>PLGSKLLLMGRSGSGKSSMRSIIFSNYSAFDTRRLGATIDVEHSHLRFLGNMTLNLWDCGGQDVFMENYFTKQKDHIFQMVQVLIHVFDVESTEVLKDIEIFAKALKQLRKYSPDAKIFVLLHKMDLVQLDKREELFQIMMKNLSETSSEFGFPNLIGFPTSIWDESLYKAWSQIVCSLIPNMSNHQSNLKKFKEIMNALEIILFERTTFLVICSSNGENSNENHDSSDNNNVLLDPKRFEKISNIMKNFKQSCTKLKSGFKTLILNNNIYVSELSSNMVCFIVLKDMNIPQELVLENIKKAKEFFQ[2x];>MVLLMGVRRCGKSSICKVVFHNMQPLDTLYLESTSNPSLEHFSTLIDLAVMELPGQLNYFEPSYDSERLFKSVGALVYVIDSQDEYINAITNLAMIIEYAYKVNPSINIEVLIHKVDGLSEDFKVDAQRDIMQRTGEELLELGLDGVQVSFYLTSIFDHSIYEAFSRIVQKLIPELSFLENMLDNLIQHSKIEKAFLFDVNSKIYVSTDSNPVDIQMYEVCSEFIDVTIDLFDLYKAPVLRNSQKSSDKDNVINPRNELQNVSQLANGVIIYLRQMIRGLALVAIIRPNGTDMESCLTVADYNIDIFKKGLED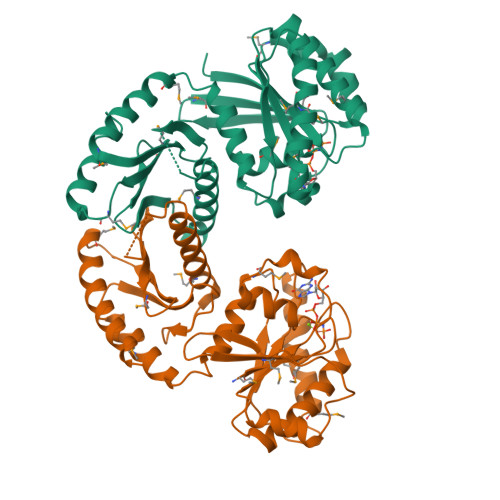IWANARASQAKNSIEDDV[2x]> MDINDKLSIDSPIDNKNIIEFITFRTDTSGIQKKIKAYQIAKHIWVVPERYYAEPLNISDEYKIDGGIYNENYLTTDKERQEYLDAICILFKRINNVIEGKKLLSLLSSASPFPFKDDTNKYLLKEALLYVNEENFEFKFFTSNIILFGPGTNISKNQVLPLNGDDATSGVGSVSEICYNPFFTKKFGEYSLDPVIGLIECLLKSLYNLYGIKVSDDIKIPYKLQRALNTDKYSYINLEEALIFGGNDYKIFTEKPYWLSNDYFLKSLNTFEENKAKYEKDLKNDPNLNNELNQYLQQKYSFSISKIWSLNLTAFADIFNINIPTSFLASITFWDRSQYYKINYPNDYNIDGFVNGQWNTNLKNIEKDNNFIIFDKPKQIITYINDIFNLRYTSNLYEDNLDIESNNYYLNFMFEYDKGNNFTINQYKALLDTLDNDFIDSLPPIQGMNAQNKLTSLPIISKGTDTENINSELLLPIHYLKSQTYNLDMYSSIKFTTNIYEVVSEKNSELVYTFLPHINEIMENYSINNTIKTEEEFYNWMENLFINYSIDILEKRNSIIPGITAVLPWIGKALNILNTNNDFEEELQLSGIKGLIKEYENFIIPDMIVPDIPLDNMPRTYDDIDKKLSEIYTKNKFLFLKGYYFIVQEWWTTYYIQFIELKYLCSGAINKQQQLLITVLEKQLFYFTNNGLFPFDAMERMINEFNRSIDIFSRISQQALNNVDIFINECALFIFNNEVYPLFLNNVENNINKANDNVLNYINKATSLTEEQIKELTVKYTFSSIAEVEFFNESYFKKITNMDIKNILTNIKNINNLILSGSQINDDITIFDESGNNLNIKFDPSIRIVDGHTNVAFKLDKSSQYINIPTENINFSFMESFSIDFWLKILDSTESTTLLNCIEDDIGWKLSIQNNNLLWEMKDNLGNNFTSLFTFNINNIWHNITLSIDRLTNTFNCFLDGKLINTDNI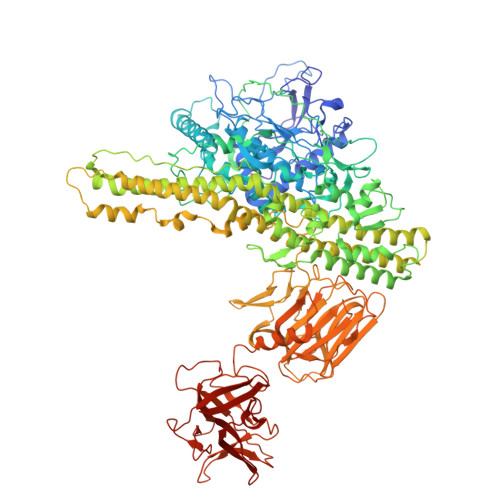SNIFSLETNTPIEIQSDNGAILLEAFSILNYPLQQQEVLNRYREAFSNNYTRNYYGDILKYNENYQLYNKTSPDKEVKKVFTNDKDYIAIEYNQNTNNPTFFSLIQKEQSKIYVEENDEVYICVQGDPLNYITIDNNQAVLTKDINLATSFKLKTNLNKPNSLIFSENSQALRLSNRLNDENYILLDLVSKLDDEPLNIFYWEFI>SSITENTSWNKEFSAEAVNGVFVLCKSSSKSCATNNLARASKEYLPASTFKIPSAIIGLETGVIKNEHQVFKWDGKPRAMKQWERDLSLRGAIQVSAVPVFQQIAREVGEVRMQKYLKKFSYGNQNISGGIDKFWLEGQLRISAVNQVEFLESLFLNKLSASKENQL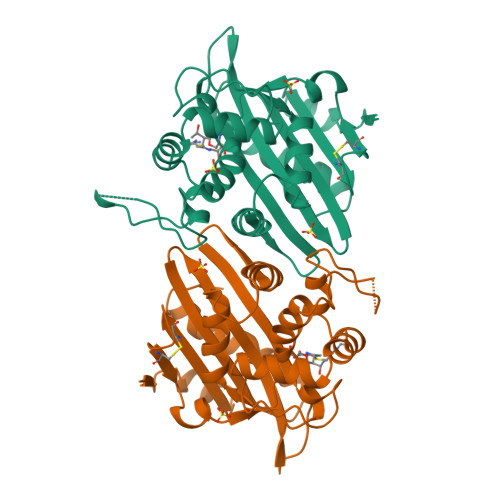IVKEALVTEAAPEYLVHSKTGFSGVGTESNPGVAWWVGWVEKGTEVYFFAFNMDIDNENKLPLRKSIPTKIMASEGIIGG[2x]> MSKIVKIIGREIIDSRGNPTVEAEVHLEGGFVGMAAAPSGASTGSREALELRDGDKSRFLGKGVTKAVAAVNGPIAQALIGKDAKDQAGIDKIMIDLDGTENKSKFGANAILAVSLANAKAAAAAKGMPLYEHIAELNGTPGKYSMPVPMMNIINGGEHADNNVDIQEFMIQPVGAKTVKEAIRMGSEVFHHLAKVLKAKGMNTAVGDEGGYAPNLGSNAEALAVIAEAVKAAGYELGKDITLAMDCAASEFYKDGKYV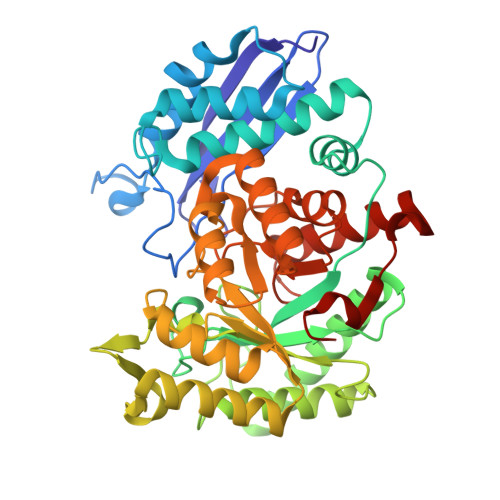LAGEGNKAFTSEEFTHFLEELTKQYPIVSIEDGLDESDWDGFAYQTKVLGDKIQLVGDDLFVTNTKILKEGIEKGIANSILIKFNQIGSLTETLAAIKMAKDAGYTAVISHRSGETEDATIADLAVGTAAGQIKTGSMSRSDRVAKYNQLIRIEEALGEKAPYNGRKEIKGQA>MDAQSSAKVNSRKRRKEVPGPNGATEEDGIPSKVQRCAVGLRQPAPFSDEIEVDFSKPYVRVTMEEACRGTPCERPVRVYADGIFDLFHSGHARALMQAKNLFPNTYLIVGVCSDELTHNFKGFTVMNENERYDAVQHCRYVDEVVRNAPWTLTPEFLAEHRIDFVAHDDIPYSSAGSDDVYKHIKEAGMFAPTQRTEGISTSDIITRIVRDYDVYAR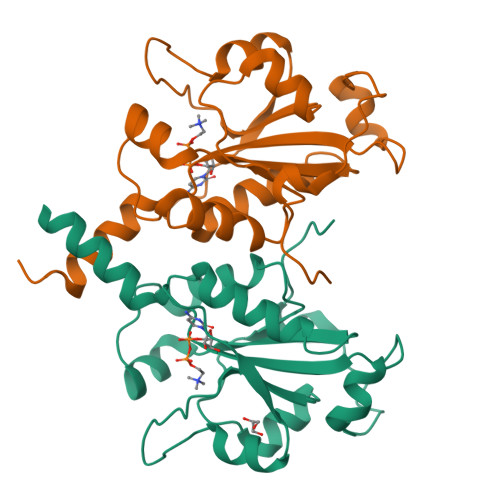RNLQRGYTAKELNVSFIN[2x]β1,3-N-acetylglucosaminyltransferases (B3GNTs) are Golgi-resident glycosyltransferases involved in the biosynthesis of poly-N-acetyl-lactosamine chains. They catalyze the addition of the N-acetylglucosamine to the N-acetyl-lactosamine repeat as a key step of the chain elongation process. Among the characterized B3GNTs, B3GNT2 is the major poly-N-acetyl-lactosamine synthase, and deletion of its coding gene dramatically reduced the cell surface poly-N-acetyl-lactosamine and led to hypersensitive and hyperresponsive immunocytes. The luminal domain of B3GNT2 comprises an N-terminal helical domain (Pro55–Cys125) and a C-terminal catalytic domain (Cys138–Cys397) as well as an extended linker (Arg126–Lys137) that connects the helical domain to the catalytic domain.

To capture the conformations of the enzyme during the entire reaction cycle, we also determined two more structures of B3GNT2: unliganded and bound to only UDP (for the state when GlcNAcβ1-3Galβ1-4GlcNAc is released). Comparison of the unliganded structure to the substrate-bound or the product-bound structure demonstrates that the substrate-binding cleft of apo B3GNT2 is available to accommodate substrates for the reaction to occur. Nevertheless, some subtle conformational changes in the cleft have been observed at different stages of the reaction cycle. One example is the catalytic residue Asp333 aforementioned. The side chain of Asp333 points away in apo B3GNT2 but rotates to engage the substrates upon binding of either the donor or the acceptor substrate. It stays engaged after the reaction and only to disengage after the release of the product GlcNAcβ1-3Galβ1-4GlcNAc.

>[4x]MHHHHHHHHENLYFQGSKEKFWKISTPPEAYWNREQEKLNRQYNPILSMLTNQTGEAGRLSNISHLNYCEPDLRVTSVVTGFNNLPDRFKDFLLYLRCRNYSLLIDQPDKCAKKPFLLLAIKSLTPHFARRQAIRESWGQESNAGNQTVVRVFLLGQTPPEDNHPDLSDMLKFESEKHQDILMWNYRDTFFNLSLKEVLFLRWVSTSCPDTEFVFKGDDDVFVNTHHILNYLNSLSKTKAKDLFIGDVIHNAGPHRDKKLKYYIPEVVYSGLYPPYAGGGGFLYSGHLALRLYHITDQVHLYPIDDVYTGMCLQKLGLVPEKHKGFRTFDIEEKNKNNICSYVDLMLVHSRKPQEMIDIWSQLQSAHLKC>MHHHHHHHMGKYDEELIKTAGTVASKGRGILAMDESNATCGKRLDSIGVENTEENRRAYRELLVTAPGLGQYISGAILFEETLYQSTASGKKFVDVMKEQNIVPGIKVDKGLVPLSNTNGESWCMGLDGLDKRCAEYYKAGARFAKW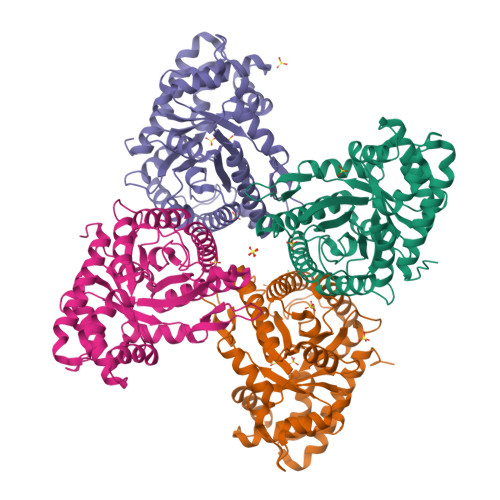RSVVSIPHGPSIIAARDCAYGLARYAAIAQNAGLVPIVEPEVLLDGEHDIDRCLEVQEAIWAETFKYMADNKVMFEGILLKPAMVTPGADCKNKAGPAKVAEYTLKMLRRRVPPAVPGIMFLSGGQSELESTLNLNAMNQSPNPWHVSFSYARALQNTVLKTWQGKPENVQAAQAALLKRAKANSDAQQGKYDATTEGKEAAQGMYEKGYVY[8x]> GAMARVTMNEFEYLKLLGKGTFGKVILVKEKATGRYYAMKILKKEVIVAKDEVAHTLTENRVLQNSRHPFLTALKYSFQTHDRLCFVMEYANGGELFFHLSRERVFSEDRARF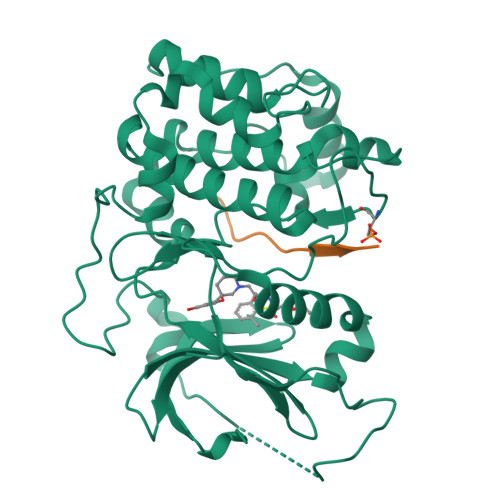YGAEIVSALDYLHSEKNVVYRDLKLENLMLDKDGHIKITDFGLCKEGIKDGATMKTFCGTPEYLAPEVLEDNDYGRAVDWWGLGVVMYEMMCGRLPFYNQDHEKLFELILMEEIRFPRTLGPEAKSLLSGLLKKDPKQRLGGGSEDAKEIMQHRFFAGIVWQHVYEKKLSPPFKPQVTSETDTRYFDEEFTAQMITITPPDQDDSMECVDSERRPHFPQFDYSASSTA;> GRPRTTSFAE> MASNNYQPASSYIQPSFAGGELAPSLQGRVDLARYAISLKTCRNFVVQPYGGASNRPGFRFNTACKYKNYATRLIPFSFNTEQTYVIEIGHQYMRFHRDGAPVLDGGEPVEVATSWHRDDIFEIKYVQSADVLTLVHPDYKPRQLKRYSETDWVLDFFDNEFGPLQDQNVDESITIISNGVVDLVELTASEAIFSEAMVGTTIKLQQVSSGEVAAWQNRSAVEQGDLAYVDERTYKATSLSGGVDNTLTGDNTPAHTEGEQWDGPRTTIQGVTETLGVKWAYLHSGFGYVRITEHRDDTHIVGRVIGRLPEEIRTEGTYRWSFAAWDSDRGYPGTASYYQQRLVFANSRAEPQAFWMSETGIFNGFKVSFPIEADDAITFTLASRQVNEIRHLIPLGSLLALTSGAEWMISDNDQGLAPDTVSADVQGYRGASDVTPLLIGSSALYVQARGTVIRDLAYSFELDGYTGDDLTIFSNHLLKDYTIKDWAYAQEPDSVVWLVRSDG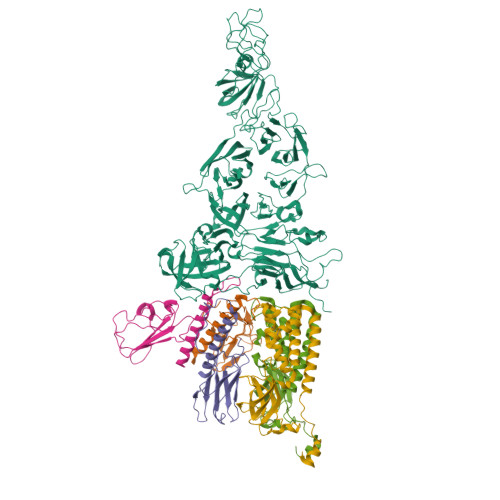ALLSMTYQREQQVVAWARHDTVDGEFESVAVIAEGSRDVPYAIVKRQVGGETVRYIEYLDSRRFSHVEDFFCVDSGLTYDGRSSTGALLTIGGGTNWTTDEDLTLTASASSFSPSDVGRRVRVYTGDKFADVDVDAYVSATSVAVSAVRIVPEELRGVQGDRWGFMAKTLTGLDHLEGKTVSILADGNVHAPEVVTGGQVTLDYSAAVVHVGLPIESDIETLPISSSGATVRDSHKAIVGVGIQLEKSRGVFAARSRRDFTSSDLIELKQRDAEDWGEATGLETGLVELGIPTSWDKDGSLFIRQSDPLPLTILSIIPRVVMGGKG;>[3x]MTVPTNDNREQYAGNGATTVFPYAFRIFESSDLEVYLTDEDGDQALLIEGTDYTVSGAGDEEGGEITFPVSGDPLDDGETLTILRVIDITQETDLKNQGAYYPEVVEDEFDRSRMIDQQQQEQLDRALIKTETGDRWEGQGVPAKNFAMSDPVEDTDLPTVRWTKDYVTQMAEGITGDIGAYTVVAPTSGDEKRLDEWMDDIQRPDDSLVVADGGTEARSLSERFADSASYQDYGIAGDGTTNDTAAFAALESDRSSDAIELHGNTYLVDEIPNGNAYRDAVWSLDGEDLSISEYGGLVTGTPTTGAFEPAYTGGVNNTPTTSGRTNKHTRAILASQNCRADFARSACVASIYSWAYGNVSGNFASRQSIAGAPQTVNIGSEEGQALGFQSGNYTTQFCRAEGSTTFNIGSDDCAASGAHSGTISSLESYAGRGHDFRGTPVFDDGVLVDITIDDAGAGYVPGSDVMYLQNRQFGNTTDAVITYTVDGTGGVSAITITDGGSGYSGIVAARIDTFGDYSLVMASARSKIEDQFCAAIASDNARVRGRESAVIASDGGVVNEDNSVVIGSVDSTSNGARSGIYTGSGCETTGAGAVVIGGVNAKASNDGAIVMGRGVDSEFARSLVFGDGGSGAAASTAGRKFQVTAAGNVTAAGTITGSTTYADYAEYFENSARGVIPLGVIVTLDGRKVRPASAGDDIIGVVSGTAILAAGDSQFHWGGRYLAGEFGELLYHDVDVDGKIERQPVENPEYDPSVPNVPRSQRPEEWSCIGLVGQLHVRVSSDVAAGDRVAAGDGGIGVPGDNGMICMEIKQAYDSGKGYAVALCLHK;>[2x]MPSKVDICNRALSNTGTDITIASLTEKSKEARLCQQWYDATLASLLRTYQWAFAQRRVTLALIGVGPAGWRHKYRYPTDAITIHDVFTADTYPDGASEFTDGRYRQIFQIASDGEGGRLVLANCEDAMCRYTSDIEDPNLMPPDFSTALEMMLAKNIAMPMTGNPGLMTVLAQQAASLVSDAIARDQNEGYRNPLPYASWTRANIGDSYPDDDHLPHRGGRR>MLAMSPPKPAVELDRHIDLDQAHAVASGGARIVLAPPARDRCRASEARLGAVIREARHVYGLTTGFGPLANRLISGENVRTLQANLVHFLASGVGPVLDWTTARAMVLARLVSIAQGASGASEGTIARLIDLLNSELAPAVPSRGTVGASGDLTPLAHMVLCLQGRGDFLDRDGTRLDGAEGLRRGRLQPLDLSHRDALALVNGTSAMTGIALVNAHACRHLGNWAVALTALLAECLRGRTEAWAAALSDLRPHPGQKDAAARLRARVDGSARVVRHVIAERRLDAGDIGTEPEAGQDAYSLRCAPQVLGAGFDTLAWHDRVLTIELNAVTDNPVFPPDGSVPALHGGNFMGQHVALTSDALATAVTVLAGLAERQIARLTDERLNRGLPPFLHRGPAGLNSGFMGAQVTATALLAEMRA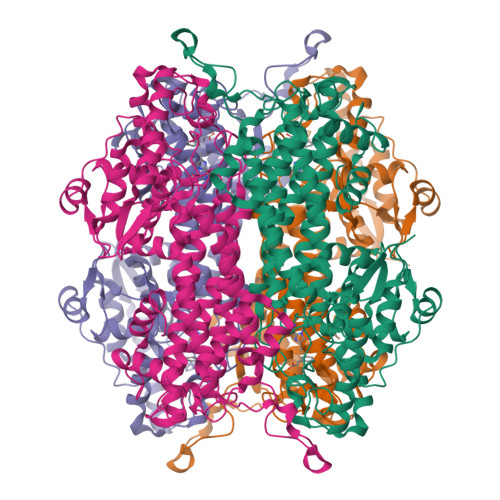TGPASIHSISTNAANQDVVSLGTIAARLCREKIDRWAEILAILALCLAQAAELRCGSGLDGVSPAGKKLVQALREQFPPLETDRPLGQEIAALATHLLQQSPV[8x]2-(1,1-difluoroethyl)-5-methyl-N-[6-(trifluoromethyl)pyridin-3-yl][1,2,4]triazolo[1,5-a]pyrimidin-7-amine | C14 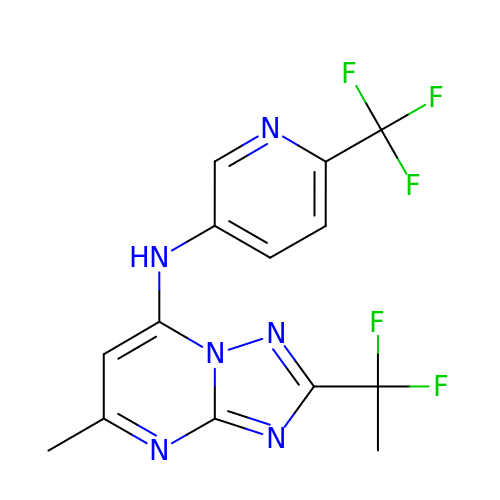H11 F5 N6 | HDLFZCDEGAWEFX-UHFFFAOYSA-N>SMSKLTKVTFIGWFKSGEMFTKDIMLSGDREEIEWVTVQLAEVNN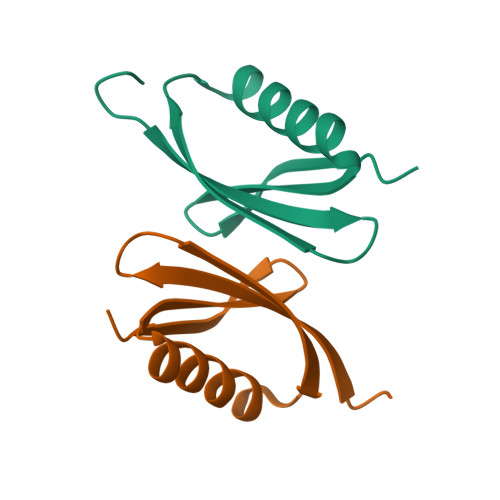ALVKAFINDEKVFEADFRG[2x]> MRWQIRKLRRAEGFNVG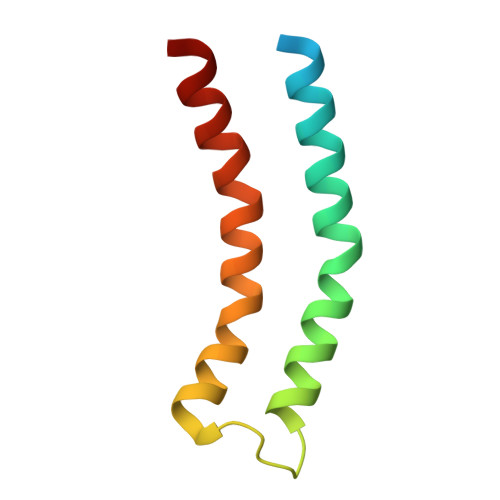LLIGLFIFILVGIVLLPVITSEVSSLTSGTSPAVTGTNATLLNLVPLFYILILVIVPAVLAYKMYRE>[4x]MEKEDSGFFSTSFKYVLSACIASFIFGYQVSVLNTIKNFIVVEFEWCKGEKDRLNCSNNTIQSSFLLASVFIGAVLGCGFSGYLVQFGRRLSLLIIYNFFFLVSILTSITHHFHTILFARLLSGFGIGLVTVSVPMYISEMTHKDKKGAYGVMHQLFITFGIFVAVMLGLAMGEGPKADSTEPLTSFAKLWWRLMFLFPSVISLIGILALVVFFKEETPYFLFEKGRIEESKNILKKIYETDNVDEPLN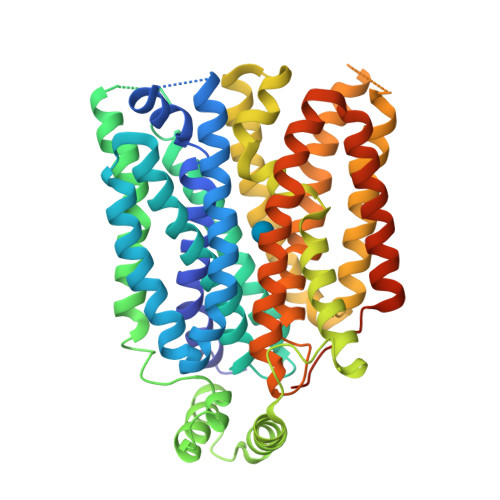AIKEAVEQNESAKKNSLSLLSALKIPSYRYVIILGCLLSGLQQFTGINVLVSNSNELYKEFLDSHLITILSVVMTAVNFLMTFPAIYIVEKLGRKTLLLWGCVGVLVAYLPTAIANEINRNSNFVKILSIVATFVMIISFAVSYGPVLWIYLHEMFPSEIKDSAASLASLVNWVCAIIVVFPSDIIIKKSPSILFIVFSVMSILTFFFIFFFIKETKGGEIGTSPYITMEERQKHMTKSVVENLYFQ>MNIEELKKQAETEIA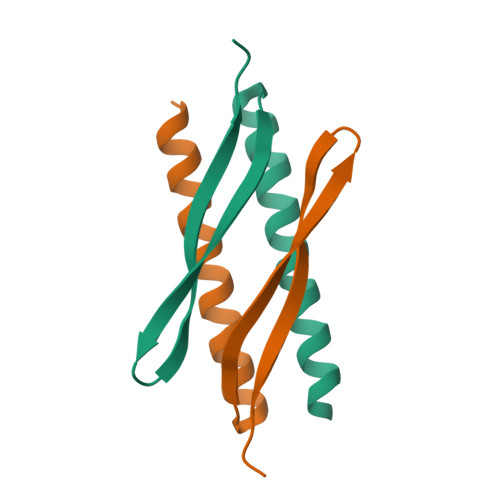DFIAQKIAELNKNTGKEVSEIRFTAREKMTGLESYDVKIKIMLEH[2x]> MAGDKGGGDGERRLRQPIVVVLGHVDHGKTTLLDKIRRTAVAAKEAGGITQHIGASIVPADVIEKIAEPLKKVIPVKLVIPGLLFIDTPGHELFSNLRRRGGSVADFAILVVDIMEGFKPQTYEALELLKERRVPFLIAANKIDRIPGWKPNPDAPFIETIRRQDPKVREILEQRVYEIVGKMYEAGLPAELFTRIKDFRRKIAIVPVSARTGEGIPELLAVLAGLTQTYLKERLRYAEGPAKGVVLEVKEMQGFGTVVDAVIYDGVLKKEDIIVVGGREGPIVTRVRALLMPAPLQDIRSREARFVQVDRVYAAAGVRIAAPGLDDVIAGSPIYAAESEEEARKLMEAVQREIEELRFRTENIGVVVKADTLGTLEALVEALRRRGVPVRLADIGPVSRSDVLDAAVTRKIDPYLGVVLAFNVKVLPEAEEEASRAGVKIFRESMIYKLIEDYEEWVKKEKEAERLKALNSLIRPGKFRILPGYVFRRSDPAIVGVEVL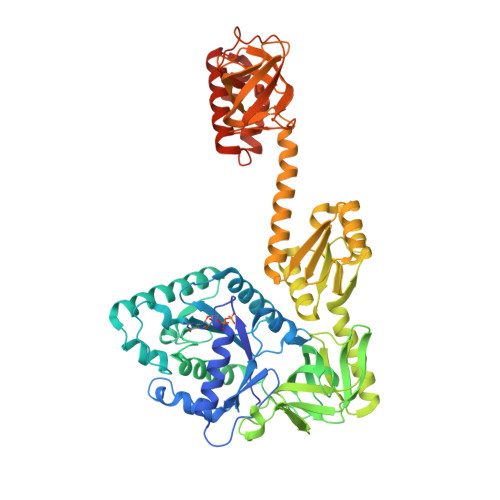GGVIRPGYPVMDSQGRELGRIMAIKDRDRSLEEARLGAAVAVSIQGRILIGRHANEGDILYTNVPAQHAYKILTEFKDLVSKDELDVLREIAEIKRRAADHEYNKVLLRLKIKRVSQHHHHHH>GRSEGALIRFYVEIEEPEKFLNCVPEELKETLLKEKRIYIDVFTTRPDTVFGATFVVLAPEHPLVPVLACIGERLGNACYSDVENFVEKMKKMSTRERTMEEDKEGVFLGVYATNPANGEKIPVWSANYVLYEYGTGAIMCVPAHDQRDWEFAKKYDLP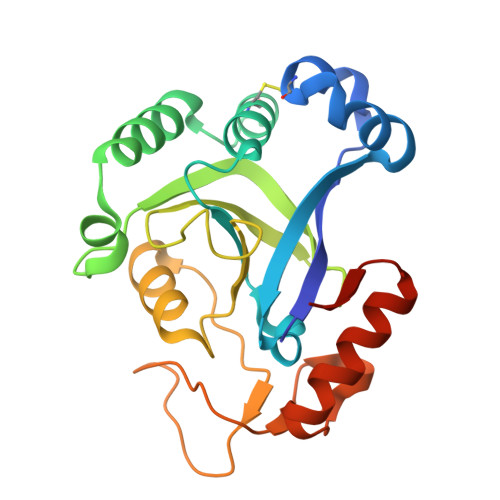IKVVVKPEGAWDFEKGAYEGKGTLVNSDGFDGLDSETAKRKITEWLQDRGLGEKKVSYRL[2x]> GSHMFFKDYQKKNVMRLLQDSLEKIINEWLKTDDESHTKLKSLQELSEMDINATSFAEHSPLPDFVTRLWLDPHKALDAMDKNISKNEIRKLIKETAREIEL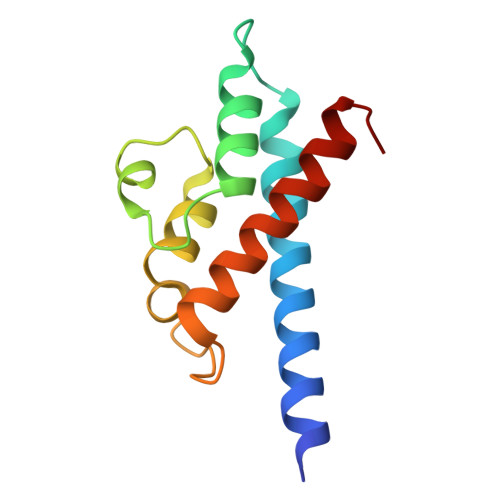VFTHQK> KFRTMRQNLQEASDVLDDQIESFTKIIQNHYKLSPNDFADPTIQSQSEIYAVGRIVPDSPTYDKFLNPESLSLETSRMGGVGRRVRLDLSQVNELSFFLGQIVAFKGKNANGDYFTVNSILPLPYPNSPVSTSQELQEFQANLEGSSLKVIVTCGPYFANDNFSLELLQEFIDSINNEVKPHVLIMFGPFIDITHPLIASGKLPNFPQFKTQPKTLDELFLKLFTPILKTISPHIQTVLIPSTKDAISNHAAYPQASLIRKALQLPKRNFKC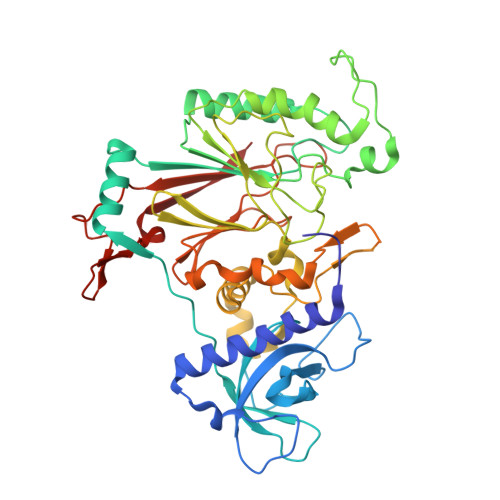MANPSSFQINEIYFGCSNVDTFKDLKEVIKGGTTSSRYRLDRVSEHILQQRRYYPIFPGSIRTRIKPKDVSTKKETNDMESKEEKVYEHISGADLDVSYLGLTEFVGGFSPDIMIIPSELQHFARVVQNVVVINPGRFIRATGNRGSYAQITVQCPDLEDGKLTLVEGEEPVYLHNVWKRARVDLIAS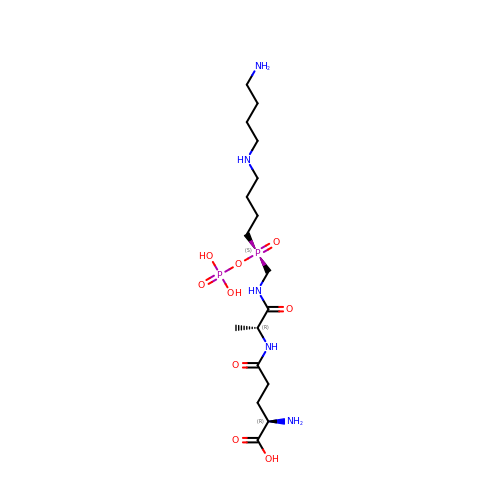D-GAMMA-GLUTAMYL-N-{[(R)-{4-[(4-AMINOBUTYL)AMINO]BUTYL}(PHOSPHONOOXY)PHOSPHORYL]METHYL}-D-ALANINAMIDE | C17 H37 N5 O9 P2 | GBZVPDJOUXPMNB-HPMPJWHZSA-N PERIDININ | C39 H50 O7 | 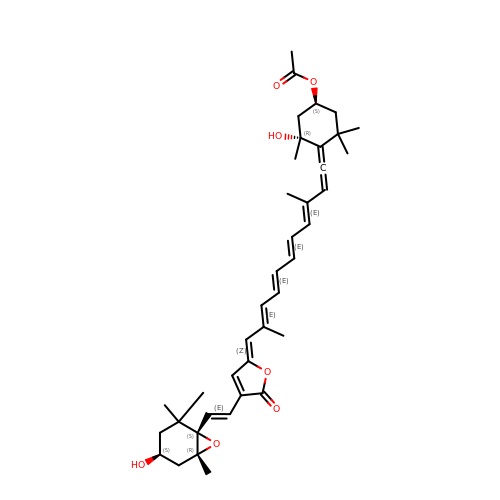UYRDHEJRPVSJFM-FROCQLDGSA-N> KFIAQRITIARAQAENLGRSEKGDFFSVKAAISFLKVDNFAYPACSNENCNKKVLEQPDGTWRCEKCDTNNARPN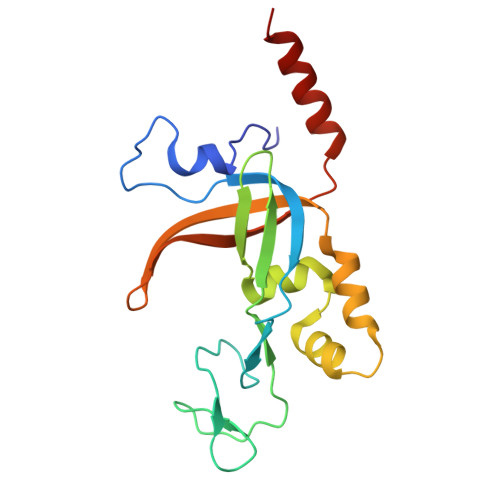WRYILTISIIDETNQLWLTLFDDQAKQLLGVDANTLMSLKEEDPNEFTKITQSIQMNEYDFRIRAREDTYNDQSRIRYTVANLHSLNYRAEADYLADELSKAL>MINNKFAVSTISDYTEKINNVKDEEVDDLIKNINKYNYDLFNGTAENQLPDYLNIHEGD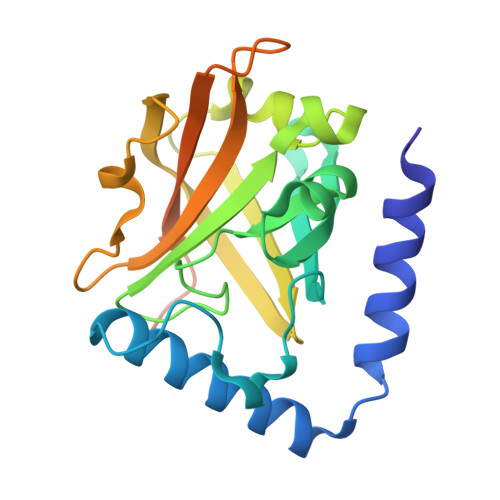VLGYIEIPSINIKLPIYYGTSVDILKKGVGVLEGTSLPVGGENTHSVLSAHTGLANQKLFTDIDKLKDGDVFYLHILKKDLAYKVNQIKVVHPDEIDELKISDDKDYVTLLTCYPYGINTERLLVRGERTDLSPSNVEQVQKEISTFNHSNENLEHHHHHH[2x]>MSSSARNTTKLKTACVTGGNGYIGSALIKMLLEEGYAVKTTVRNPDDMEKNSHLKGLQELGPLTVLRADMDEEGSLDDAVAGCDYAFLVAAPVNLWAQDPEKQQIEPSVRGTLNAVRSCVKAGTVRRVILTSSAAGVYIRPDLQGDGHALDEDSWSDVDFLRANKPPTWGYCVSKVLLEKAACRFAEEHGISLVTVCPVLTVGAAPAPKVRTSIVDSLSMLSGDEAGLAVLRGIETTSGALQLVHIDDLCRAELFLAEEAAAGGRYICCSLNTTVVELARFLAHKYPQYRVKTNFDDDEHLLERPRVIMSSEKLVREGFEYRHNTLDEIYDNVVEYGKALGILPY[2x]

Dihydroflavonol 4-reductase (DFR) and flavanone 4-reductase (FNR) reduce dihydroflavonols and flavanones, respectively, using NAD(P)H to produce flavan-(3)-4-(di)ols in flavonoid biosynthesis. Anthocyanidin reductase (ANR) reduces anthocyanidins to flavan-3-ols. In addition to their sequences, the 3D structures of recombinant DFR, FNR and ANR from sorghum and switchgrass showed a high level of similarity. The catalytic mechanism, substrate-specificity and key residues of three reductases were deduced from crystal structures, site-directed mutagenesis, molecular docking, kinetics, and thermodynamic ana-lyses.

The position and orientation of bound naringenin in the ternary complex structure of SbFNR2 did not favor its catalytic reaction. The C4 atom of the naringenin carbonyl group was 5 Å away from C4 of NADP+ and its oxygen was not hydrogen bonded to any of the catalytic triad residues, which is consistent with the lack of activity observed with this substrate in SbFNR2. The para-hydroxyl group on the B-ring of naringenin was hydrogen-bonded to the phenolic side chain of Tyr-138 and the backbone amide of Leu-200. The same hydroxyl group was also connected to the backbone and side chain of Gln-242 through a water molecule. The hydroxyl group on C5 of the A-ring established a direct hydrogen bond with the side chain of Thr-212 and an indirect hydrogen bond with the pyrophosphate group of NADPH through a water molecule. C7 of the A-ring was also hydrogen bonded with the side chain of Asp-216 and the backbone amide of Thr-212. SbFNR2 and SbANR did not display any activity against naringenin and eriodictyol despite substantially longer reaction times. In addition, both SbFNR1 and SbFNR2 displayed ANR activity, reducing cyanidin and pelargonidin to epicatechin and epiafzelchin, respectively. It is especially noteworthy that the activity of SbFNR2 against epiafzelchin reaches 43% of SbANR activity.>[4x]MHNVLIVGASR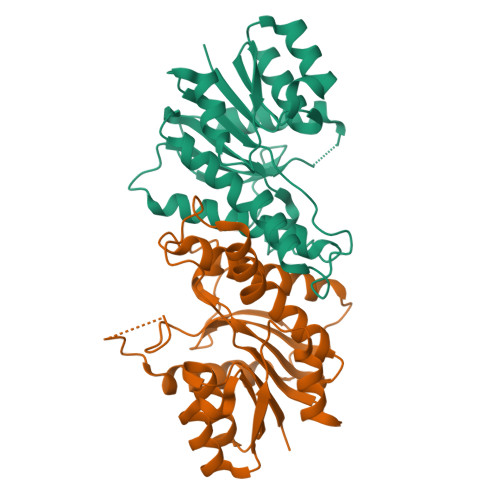GIGLGLADAFLQRGAQVFAVARRPQGSPGLQALAERAGERLQAVTGDLNQHDCAERIGEMLGERRIDRLIVNAGIYGPQQQDVAEIDAEQTAQLFLTNAIAPLRLARALSGRVSRGGVVAFMSSQMASLALGLSATMPLYGASKAALNSLVRSWEGEFEELPFSLLLLHPGWVRTEMGGDSAPLSVEESAAGLVAAVEDAAGVNACRFVDYRNQPLPW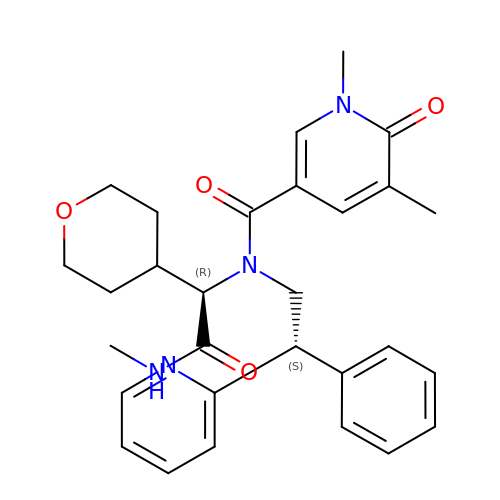1,5-dimethyl-~{N}-[(1~{R})-2-(methylamino)-1-(oxan-4-yl)-2-oxidanylidene-ethyl]-6-oxidanylidene-~{N}-[(2~{S})-2-phenyl-2-pyridin-2-yl-ethyl]pyridine-3-carboxamide | C29 H34 N4 O4 | MDCZQITXTAMNNV-AOYPEHQESA-N>GSMERKRWECPALPQGWEREEVPRRSGLSAGHRDVFYYSPSGKKFRSKPQLARYLGGSMDLSTFDFRTGKM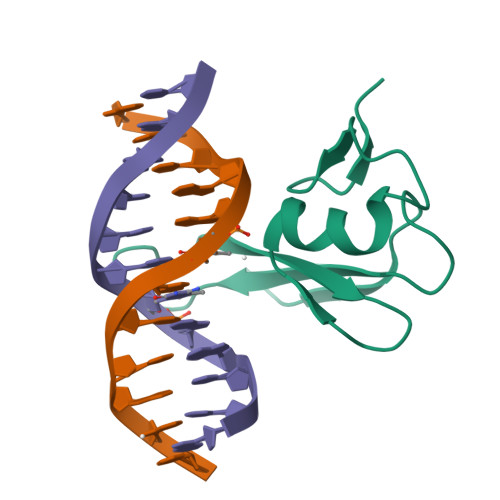LM[2x]For instance, polo-like kinase 1 (Plk1, a member of five Plks), a validated anticancer target, has a unique exterior surface (polo-box domain, PBD) composed of charged, hydrophobic, and hydrophilic domains whose phosphorylation-dependent protein-protein interactions are crucial in regulating mitotic progression and cell proliferation. A large body of evidence suggests that PBD interacts with phosphoserine/phosphothreonine (pS/pT)-containing motifs, and directs the N-terminal catalytic activity to specific subcellular localizations. The polo-box domain consists of two different binding regions, such as the unique, broader pyrrolidine-binding pocket and the conserved, narrow, Tyr-rich hydrophobic channel, among the three Plk polo-box domains (Plks 1–3), respectively. The N-terminal Pro residue on PLHSpT is crucial in conferring specificity by docking its side chain into a unique hydrophobic core (hereafter called the pyrrolidine-binding pocket), which is surrounded by the Trp414, Phe535, and Arg516 residues.

Our assay results revealed that the peptide-containing adamantyl group at the N-terminus (PL-55) showed one of the highest binding affinities, compared to PL-42. Finally, in an attempt to determine the molecular basis for the enhanced binding affinity on PL-55, we solved the co-crystal structure of Plk1 PBD in complex with PL-55. More importantly, the crystal structure of Plk1 PBD in complex with PL-55 further reinforces our detailed understanding of the unique binding nature of the pyrrolidine-binding region, showing that the hydrophobic interactions between the adamantyl moiety and the unprecedented, new PBD-interacting elements, such as Arg518 and Gln536, played an important role for the specific tight binding into the broad, pyrrolidine hydrophobic pocket. Notably, the side-chain conformation of Arg518 rotated by around 120 degrees to accommodate the hydrophobic adamantyl moiety presented to the pocket. Furthermore, the above two PBD residues were either not identified in the previous crystal studies due to the high flexibility, or they reside in the reverse direction of the peptide chain. Thus, the crystal data indicated that the bulky adamantyl substitution in PL-55 acted as a site-directed moiety that prevented the N-terminal Pro motif from turning into the narrow passage of the Tyr-rich hydrophobic channel. Moreover, in contrast to the dual-binding ability of PL-49, PL-55 could not provide the additional hydrophobic interactions from the Tyr-rich hydrophobic channel; thus, PL-55 showed a small decrease in potency. As expected, PL-42 and PL-55, having bulky N-terminal substituents like trimethoxy-substituted benzyl or the adamantyl group, buried into the broader pyrrolidine-binding pocket, which was confirmed using X-ray crystallography, and has been shown to participate with the newly identified unique PBD residues that mediate hydrophobic interactions.

> CHLSDMLQQLHSVNASKPSERGLVRQEEAEDPACIPIFWVSKWVDYSDKYGLGYQLCDNSVGVLFNDSTRLILYNDGDSLQYIERDGTESYLTVSSHPNSLMKKITLLKYFRNYMSEHLLKAGANITPREGDELARLPYLRTWFRTRSAIILHLSNGSVQINFFQDHTKLILCPLMAAVTYIDEKRDFRTYRLSLLEEYGCCKELASRLRYARTMVDKLLSS5-[2-(TRIFLUOROMETHOXY)PHENYL]-2-FUROIC 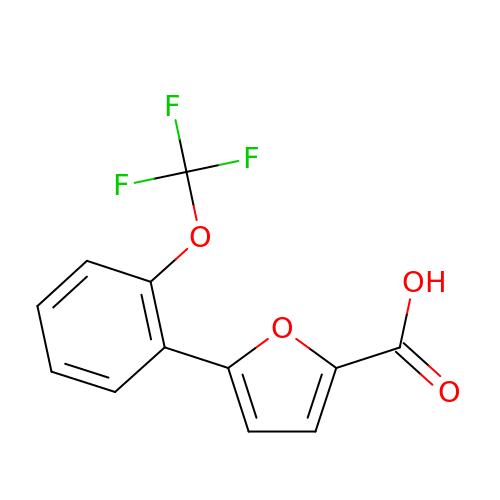ACID | C12 H7 F3 O4 | PSLFQKRPFOCZHR-UHFFFAOYSA-N>MSLRYTKEQCTAAEAQRLAQEIAFGPVVFQVSRLMLKFGIFQLLSGKREGYTLQEISGRTGLTRYAAQVLLEASLTIGTILLEEDRYVLAKAGWFLLNDKMARVNMEFNHDVNYQGLFHLEEALLNGRPEGLKVFGEWPTIYEGLSQLPEQVQKSWFGFDHFYSDQSFGKALEIVFSHHPKRLLDIGGNTGK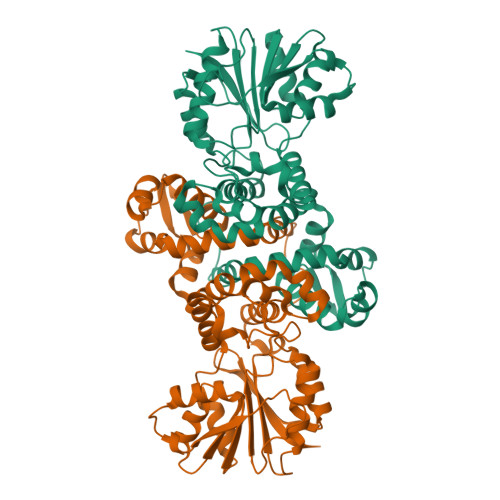WATQCVQYNKEVEVTIVDLPQQLEMMRKQTAGLSGSERIHGHGANLLDRDVPFPTGFDAVWMSQFLDCFSEEEVISILTRVAQSIGKDSKVYIMETLWDRQRYETASYCLTQISLYFTAMANGNSKMFHSDDLIRCIENAGLEVEEIQDNIGLGHSILQCRLKEGHHHHHH[2x]> MASMKKKGSVVIVGRVVLSGGSGDTAYAQQTRGEESTQETSQTGRDTNENCGEVQVLS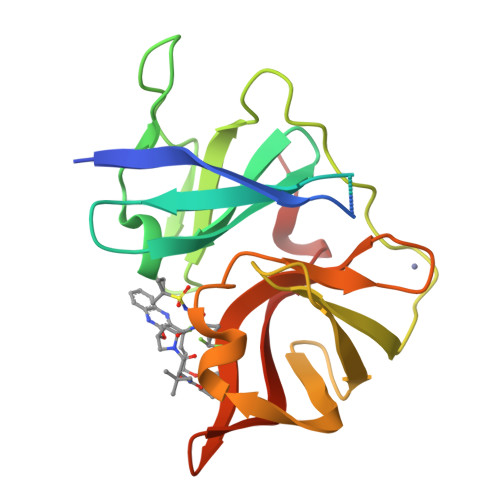TATQSFLGTAVNGVMWSVYHGAGGKTISGPKGPVNQMYTNVDQDLVGWPAPPGVKSLTPCTCGASDLYLVTRHADVVPVRRRGDTRGALLSPRPISTLKGSSGGPLLCPMGHVAGLFRAAVCTRGVAKAVDFVPVESLETTMRSP>[2x]MRSRRVDVMDVMNRLILAMDLMNRDDALRVTGEVREYIDTVKIGYPLVLSEGMDIIAEFRKRFGCRIIANFKVADIPETNEKICRATFKAGADAIIVHGFPGADS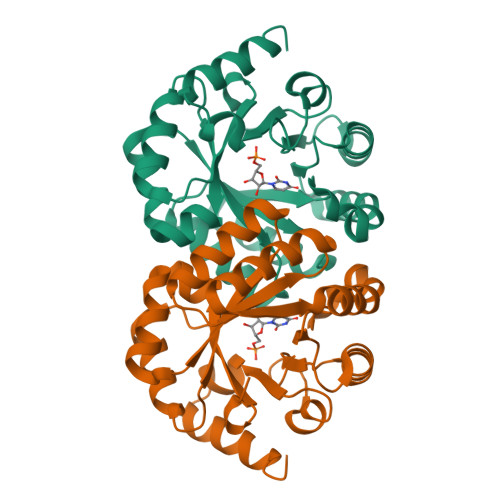VRACLNVAEEMGREVFLLTEMSHPGAEMFIQGAADEIARMGVDLGVKNYVGPSTRPERLSRLREIIGQDSFLISPGVGAQGGDPGETLRFADAIIVGRSIYLADNPAAAAAGIIESIKDLLNP> NLINFMEMIRYTIPCEKTWGEYADYGCYCGAGGSGRPIDALDRCC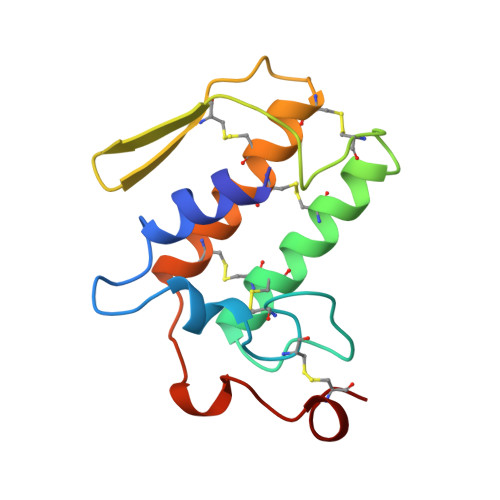YVHDNCYGDAEKKHKCNPKTQSYSYKLTKRTIICYGAAGTCARIVCDCDRTAALCFGNSEYIEGHKNIDTARFCQ Thioredoxin (Trx), glutaredoxin (Grx), and peroxiredoxin (Prx) are redoxin proteins that are important in regulating a variety of cell redox-related processes. BNP7787 (Tavocept, Disodium-2,2'-dithio-bis-ethanesulfonate) is a novel, water soluble disulfide that has been evaluated in oncology-related clinical studies, and interaction of BNP7787 with different redoxin proteins has been a focus of research in our laboratory. Herein, structure function data including activity assays, mass spectrometry characterizations, and X-ray crystallographic studies, elucidating interactions between BNP7787 and human Grx 1, human Prx 1, and human Prx 4 are presented. These data characterize covalent BNP7787-derived mesna moieties on cysteine residues of human Grx 1, Prx 1, and Prx 4 and provide information about the functional consequences of BNP7787-mediated modifications.

Grx is a small glutathione-dependent protein, which maintains a reduced state of cysteines in cellular proteins, and is primarily involved in catalyzing the reduction of glutathione mixed disulfides and producing glutathione disulfide as a by-product. A high resolution crystal structure was solved showing the atomic interactions between Grx 1 and BNP7787. The Grx-BNP7787 co-crystal crystallizes as a monomer in the asymmetric unit. BNP7787-derived mesna moieties were observed as mixed disulfides on Cys 7 and Cys 82. Both cysteines that interact with BNP7787 (Cys 7 and Cys 82) are solvent accessible. The BNP7787-derived mesna adducts on Grx 1 are located at a crystal contact and within close proximity of each other (data not shown). Specifically, X-ray crystallography data herein shows that two of the five cysteines present in Grx 1 were modified, Cys 7 and Cys 82. Cys 22 and Cys 25 (active site residues) and Cys 78 were not modified.

> GAGTAQEFVNCKIQPGKVVVFIKPTCPYCRRAQEILSQLPIKQGLLEFVDITATNHTNEIQDYLQQLTGARTVPRVFIGKDCIGGCSDLVSLQQSGELLTRLKQIGALQ pmcAlcohol dehydrogenases (ADHs EC 1.1.1.1) are NAD(P)H‐dependent medium‐chain oxidoreductases found in all kingdoms of life. These enzymes typically catalyse the reversible reduction of aldehydes or ketones to the corresponding alcohol. The structural motifs of ADHs are highly conserved in all known eukaryotic examples; most notably, a zinc ion involved in catalysis, a second zinc ion involved in maintaining protein structure, and the Rossmann peptide‐fold involved in cofactor binding. ADHs have been shown to catalyse many complex biochemical transformations in plant natural product biosynthesis, suggesting that their catalytic repertoire has been expanded.

We also report the structure of the ADH geissoschizine synthase (GS) that catalyses an atypical 1,2‐iminium reduction. GS catalyses the irreversible 1,2‐iminium reduction of strictosidine aglycone to form geissoschizine, another intermediate in vinblastine biosynthesis. GS and THAS (47.7 % and 53.8 % amino acid identity to DPAS respectively) each crystallised with both the catalytic and structural zinc ions bound. Mutagenesis of GS residues involved in the coordination of the catalytic zinc (His73 and Cys168) resulted in the abolishment of GS activity, suggesting that, as in the canonical ADH mechanism, the catalytic zinc is essential for 1,2‐reduction of the iminium. Additionally, GS and THAS each had mutations in highly conserved residues involved in the proton relay observed in canonical ADH reduction. Moreover, GS contains a Phe residue in this position (Phe53). No substantial change in reduction activity was observed for GS Phe53Tyr mutant or the corresponding THAS Tyr56Phe mutant, suggesting the hydroxyl‐group has no catalytic role. Although THAS Glu59 is positioned 3.6 Å from the 2′O of bound‐NADP+, GS Glu56 is positioned 7.6 Å from this moiety which is not consistent with a role for this residue in cofactor binding or catalysis. GS has been reported to be able to reduce precondylocarpine acetate, albeit it at substantially reduced efficiency compared to DPAS.

>GPAGETTKLDLSVKAVGWGAADASGVLQPIKFYRRVPGERDVKIRVLYSGVCNFDMEMVRNKWGFTRYPYVFGHETAGEVVEVGSKVEKFKVGDKVAVGCMVGSCGQCYNCQSGMENYCPEPNMADGSVYREQGERSYGGCSNVMVVDEKFVLRWPENLPQDKGVALLCAGVVVYSPMKHLGLDKPGKHIGVFGLGGLGSVAVKFIKAFGGKATVISTSRRKEKEAIEEHGADAFVVNTDSEQLKALAGTMDGVVDTTPGGRTPMSLMLNLLKFDGAVMLVGAPESLFELPAAPLIMGRKKIIGSSTGGLKEYQEMLDFAAKHNIVCDTEVIGIDYLSTAMERIKNLDVKYRFAIDIGNTLKFEE[2x]>NLIQDKQTDFGLQVFAEAVQSAPDRNLALSPYGIASVLGMAQMGAYGATLKLLASKMGYSLQERGMPKLQRLLQRDLASEDGVEVASGVMVDRKIILEKVFRRSLSKAFQSVPHQIDFSQPEMARQVINSWTSDHTDGMISEFLPSGVLSELTRLVFLNALHFHGVWKTPFDPRNTREQLFHTVNGSAVSVPMMTTTQKFNYGEFVSKDGVDYDVIEMPYEGESISMLLVTPFEKDVPLSALNKELSSSRIHQWRQEMRKISKQLSIPRFSMDTEIDLKSTLSRMGLGDIFSQSRADFSRITTEEPLCVSKVLQRVKLEVNEEGT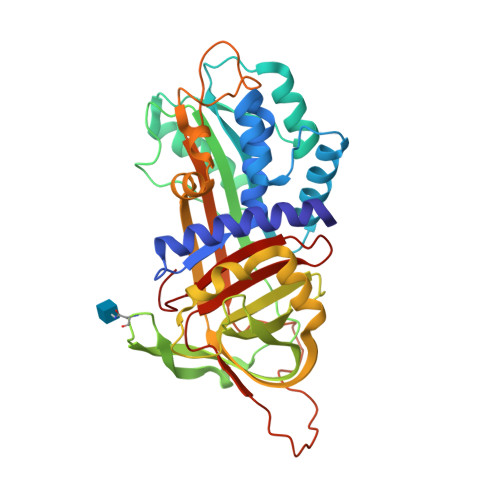KGSSATAAVIYSRMAVEEITLDRPFFFLIQHKPTGALLFSGQLTQPQEY[2x]>MSSVLVLGRISDDPASHYEQLKPLLDYVVPRMREVGIRRGEILMAPDARQMSSYLRRGRVDWVSETTGAAMLLEQRGSAHPLLMTERGGLRDFHTLFFVRRDSPIHSLSQLRGHTLALQNASSTSGYLLPMLELLRNGIACDVLLSADDTPARGSAGYLMVGSKLNVAAFVHKHLIDVGALSNVDWDDERHMPPVFKRDFRIVHRTAPVPRAVEMVRTGMDPAVEQRLRVVLLQAASDPKAGPALKRFFDTTGFRPLDP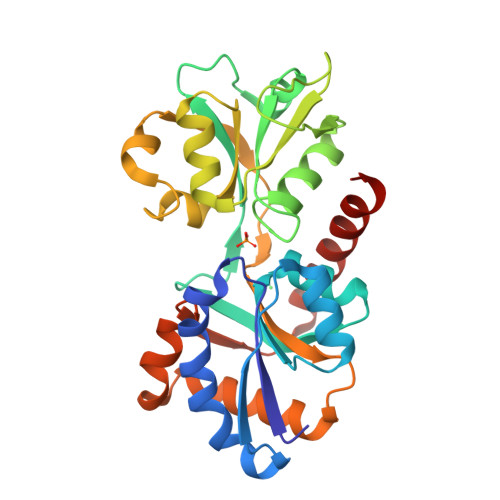TSRRRLQELSAGVQRVRDHVE[2x]>HHHHHHMASSAQDGNNPLFSPYKMGKFNLSHRVVLAPMTRCRALNNIPQAALGEYYEQRATAGGFLITEGTMISPTSAGFPHVPGIFTKEQVREWKKIVDVVHAKGAVIFCQLWHVGRASHEVYQPAGAAPISSTEKPISNRWRILMPDGTHGIYPKPRAIGTYEISQVVEDYRRSALNAIEAGFDGIEIHGAHGYLIDQFLKDGINDRTDEYGGSLANRCKFITQVVQAVVSAIGADRVGVRVSPAIDHLDAMDSNPLSLGLAVVERLNKIQLHSGSKLAYLHVTQPDYVAYGQTEAGRLGSEEEEARLMRTLRNAYQGTFICSGGYTRELGIEAVAQGDADLVSYGRLFISNPDLVMRIKLNAPLNKYNRKTFYTQDPVVGYTDYPFLQGNGSNGPLSRL[2x]

Jasmonates are phytohormones that are pivotal in mediating plant responses to various biotic and abiotic stresses and regulating plant growth. The first crystal structure of OPR3 from tomato (SlOPR3) showed that the enzyme crystallized as a self-inhibitory dimer in which the L6 loop, a critical loop involved in substrate recognition and coenzyme binding, from each protomer intrudes into the active site cavity of the other protomer. Based on these observations, it was postulated that the formation of the self-inhibitory homodimer represents a mechanism for regulating OPR3 activity and, thereby, jasmonic acid biosynthesis.

Like in the case of R283E, the monomeric structure of R283D is nearly identical to that of the wild type (RMSDCα = 0.32 Å), with loop L6 almost entirely missing because of disorder. Structurally, it is unclear why R283E prefers to crystallize in its monomeric form while R283D prefers the dimeric form. Nevertheless, our crystallographic data show that substituting R283 for an oppositely charged residue generally affects L6 conformation and thus the dimerization process. Regarding the variants, the results show that substituting residues R283 and Y364 had no significant effect on the enzyme's behavior during gel filtration.>MALRADQVSLIGQVFESYLLQHHRDDILGILRQGDDEAHYPVLVDALTLFETNMEIGEYFNAFPSQVLPIFDGALRRAAMAVLQAATPSPELRMKPNLHARISGLPICPELTREHIPKTRDVGHFLSVTGTVIRTSLVKVLEFERSYICNKCKHVFVAKADFEQYYAFCRPSACLNEEGCNSTKFTCLSGTSSSP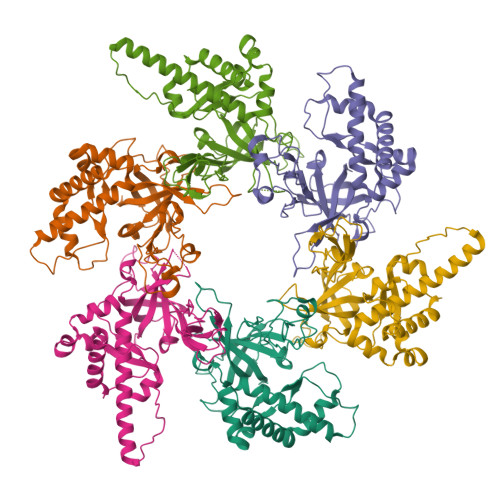SSCRDYQEIKIQEQVQRLSVGSIPRCMVVVLEDDLVDSCKSGDDITVYGVVMQRWKPFHQDARCDLELVLKANYVKVN[3x];>ASSRLVQSTLDQFIPYKGWKLYFSEAYADKSPFVQKTQAFEKFFMQRIELYDKDEIERKGSILVDYKELIEDRELTKSIPNISTELRDMPQKILQCMGLAIHQVLTKDLERHAAELQVQEGLPLDGEPIINVPLIHARLYNYEPLTQLKNVRANCYGKYIALRGTVVRVSNIKPLCTKLAFVCGTCGDVQSVPLPDGKYTLPTKCLVPECRGRSFTPDRSSPLTATVDWQSVKVQELMSDDQREAGRIPRTIECELVQDLVDSCVPGDVVTITGVVKVSSTEEGASKNKNDKCVFLLYIEANSVSNSK[3x]>SNAMTTANTPVRPKSAIDAVADAYTEKLIELNPSFATTLGLPGHETEYQDYSPAGAAAHAEATRLALEALAGLEPSDDVDAVTLDAMRERLGLELEIHQSGWDAADLNNIASPAQDIRAIFDLMPTDTVEHWEHIAGRAANVPGAIEGYIASLRAAKDDRKVAAARQIRIVIEQTGRYAAEDGFFAKMAADASLGDAPLPAEVQDKLDAGTSAARSAYSALGAFLRDELLPVAPEKDAVGRERYSLASRSFIGAEVDLEETYAWGVQELERLISEQEKVAGQIKPGASIEEAKSILNNDPARQIKGTDALKAWMQELSDRAVSELADVHFDIPDVMKTLECMIAPTDEGGIYYTGPSDDFSRPGRMWWSVPAGEDTFTTWSETTTVFHEGVPGHHLQVATATYRRELLNNWRRNVCWVSGHGEGWALYAEQLMLELGYLKDPGDHMGMLDGQRMRAARVVFDIGVHLELPVPERWGTGTWTPEKGFDFLKANLDISEGQLQFEFTRYLGWPGQAPSYKVGQRLWEQIRAELESREGFDLKSFHSKALNIGSVGLDVLRRALL[2x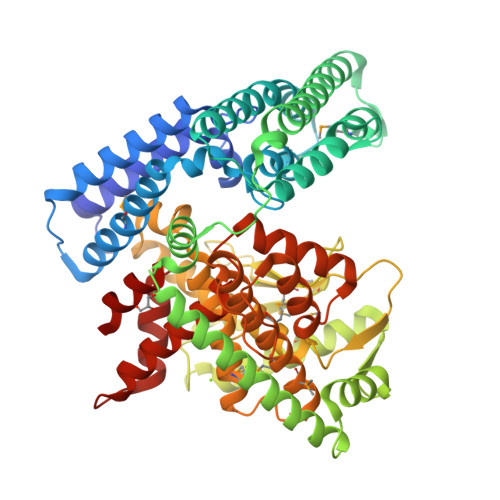]>[2x]LTLGNTTSSVILTNYMDTQYYGEIGIGTPPQTFKVVFDTGSSNVWVPSSKCSRLYTACVYHKLFDASDSSSYKHNGTELTLRYSTGTVSGFLSQDIITVGGITVTQMFGEVTEMPALPFMLAEFDGVVGMGFIEQAIGRVTPIFDNIISQGVLKEDVFSFYYNRDSENSQSLGGQIVLGGSDPQHYEG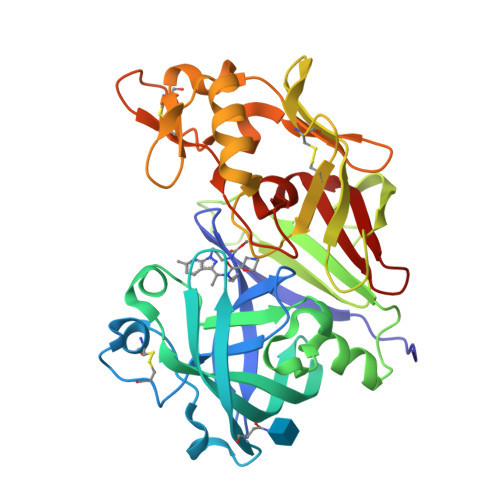NFHYINLIKTGVWQIQMKGVSVGSSTLLCEDGCLALVDTGASYISGSTSSIEKLMEALGAKKRLFDYVVKCNEGPTLPDISFHLGGKEYTLTSADYVFQESYSSKKLCTLAIHAMDIPPPTGPTWALGATFIRKFYTEFDRRNNRIGFALAR>MADAAPQLGKRKRELDVEEAHAASTEEKEAGVGNGTCAPVRLPFSGFRLQKVLRESARDKIIFLHGKVNEASGDGDGEDAVVILEKTP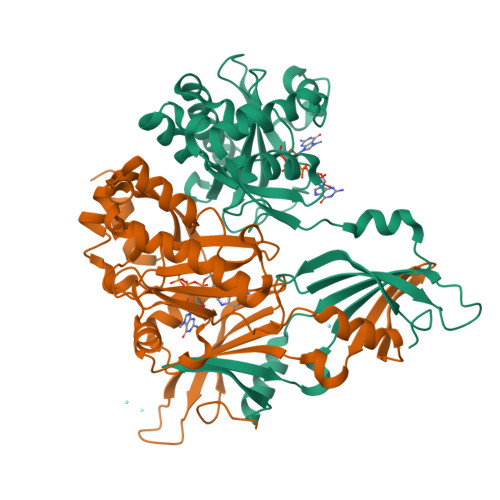FQVEQVAQLLTGSPELQLQFSNDIYSTYHLFPPRQLNDVKTTVVYPATEKHLQKYLRQDLRLIRETGDDYRNITLPHLESQSLSIQWVYNILDKKAEADRIVFENPDPSDGFVLIPDLKWNQQQLDDLYLIAICHRRGIRSLRDLTPEHLPLLRNILHQGQEAILQRYRMKGDHLRVYLHYLPSYYHLNVHFTALGFEAPGSGVERAHLLAEVIENLECDPRHYQQRTLTFALRADDPLLKLLQEAQQS[2x]> MSSVTWAP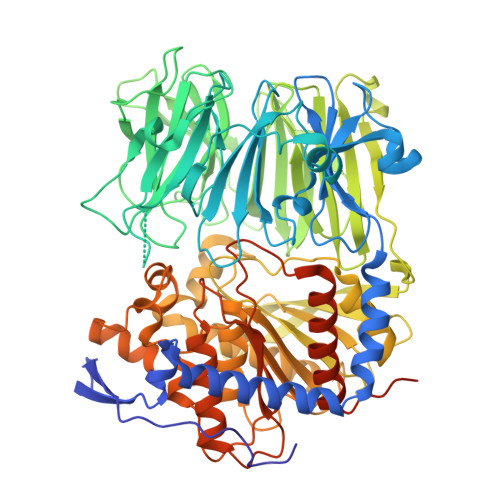GNYPSTRRSDHVDTYQSASKGEVPVPDPYQWLEESTDEVDKWTTAQADLAQSYLDQNADIQKLAEKFRASRNYAKFSAPTLLDDGHWYWFYNRGLQSQSVLYRSKEPALPDFSKGDDNVGDVFFDPNVLAADGSAGMVLCKFSPDGKFFAYAVSHLGGDYSTIYVRSTSSPLSQASVAQGVDGRLSDEVKWFKFSTIIWTKDSKGFLYQRYPARERHEGTRSDRNAMMCYHKVGTTQEEDIIVYQDNEHPEWIYGADTSEDGKYLYLYQFKDTSKKNLLWVAELDEDGVKSGIHWRKVVNEYAADYNIITNHGSLVYIKTNLNAPQYKVITIDLSKDEPEIRDFIPEEKDAKLAQVNCANEEYFVAIYKRNVKDEIYLYSKAGVQLTRLAPDFVGAASIANRQKQTHFFLTLSGFNTPGTIARYDFTAPETQRFSILRTTKVNELDPDDFESTQVWYESKDGTKIPMFIVRHKSTKFDGTAAAIQYGYGGFATSADPFFSPIILTFLQTYGAIFAVPSIRGGGEFGEEWHKGGRRETKVNTFDDFIAAAQFLVKNKYAAPGKVAINGASNGGLLVMGSIVRAPEGTFGAAVPEGGVADLLKFHKFTGGQAWISEYGNPSIPEEFDYIYPLSPVHNVRTDKVMPATLITVNIGDGRVVPMHSFKFIATLQHNVPQNPHPLLIKIDKSWLGAGMGKPTDKNVKDAADKWGFIARALGLELKTVEMFDTNATRLPIWGIGCNPWTAEHVDQTLASGNDIC(2E,6E,10E,14E,18E,22E,26E)-3,7,11,15,19,23,27,31-OCTAMETHYLDOTRIACONTA-2,6,10,14,18,22,26,30-OCTAENYL TRIHYDROGEN DIPHOSPHATE | 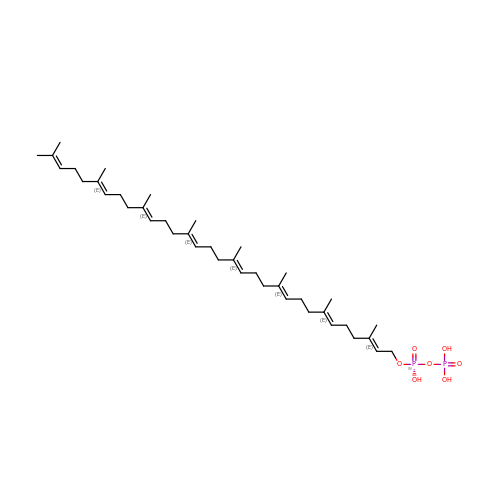C40 H68 O7 P2 | IKKLDISSULFFQO-DJMILUHSSA-N>GSMGGEVQNMLEGVGVDINKALLAKRKRLEMYTKASLKTSNQKIEHVWKTQQDQRQKLNQEYSQQFLTLFQQWDLDMQKAEEQEEKILNMFRQQQKILQQSRIVQSQRLKTIKQLYEQFIKSMEELEKNHDNLLTGAQNEFKKEMAMLQKKIMMETQQQEIASVRKS[8x]

Synapsis is achieved by the assembly of an elegant molecular structure, the synaptonemal complex (SC), which acts as a ‘zipper’ to bring in close apposition pairs of homologous chromosomes. According to this initial map of the SC, the SYCE1, SYCE2, SYCE3 and TEX12 proteins form the central element, whilst SYCP2 and SYCP3 are the main constituents of the lateral element (Costa et al., 2005; Hamer et al., 2006; Schramm et al., 2011). We determine that SYCP3 is a tetrameric protein and that its helical core folds in an elongated rod-like structure spanning 20 nm in length. We conclude that concurrent DNA-binding and higher order assembly by SYCP3 on meiotic chromosomes lead to compaction and organisation of the chromosome axis, in a manner conducive to SC central region assembly, recombination and crossover formation.

We thus identified a core region of human SYCP3, corresponding to amino acids 66–230 (SYCP3Core), that is highly stable and can be purified in large quantities to near homogeneity. The crystals contain two tetramers in the asymmetric unit; the tetramers are almost identical both between and within iodide derivative and native structures. The overall architecture of SYCP3 is an extended rod-like structure that spans approximately 20 nm in length. The helical chains of the SYCP3 tetramer are arranged in an alternating anti-parallel fashion, such that each end of the tetramer contains two N-termini and two C-termini. The SYCP3 structure undergoes a left-handed 90° rotation along its length so that the two N-termini at each end of the tetramer lie in orthogonal planes. The two halves of the structure (hereafter referred to as arms) are formed of a four-helix bundle leading into a coiled-coil that zips together the C-terminal parallel chains, leaving the N-terminal ends to splay apart. The most prominent structural feature driving the tetrameric assembly of SYCP3 chains is the presence of two four-helix bundles, one in each arm of the tetramer. The centre of the SYCP3 tetramer is intrinsically asymmetrical as parallel chains B and D interact in a coiled-coil, keeping chains A and C apart by steric exclusion. Instead, the central region likely oscillates between two conformations, in which the coiled-coil encompasses either chains B and D or chains A and C. In both conformations, the left-handed 90° rotation would be retained; interchange between conformations would require a transitory super-helical unwinding of the central region.>AEEFPVPNGFESAYREVDGVKLHYVKGGQGPLVMLVHGFGQTWYEWHQLMPELAKRFTVIAPDLPGLGQSEPPKTGYSGEQVAVYLHKLARQFSPDRPFDLVAHDIGIWNTYPMVVKNQADIARLVYMDAPIPDARIYRFPAFTAQGESLVWHFSFFAADDRLAETLIAGKERFFLEHFIKSHASNTEVFSERLLDLYARSYAKPHSLNASFEYYRALNESVRQNAELAKTRLQMPTMTLAGGGHGGMGTFQLEQMKAYAEDVEGHVLPGC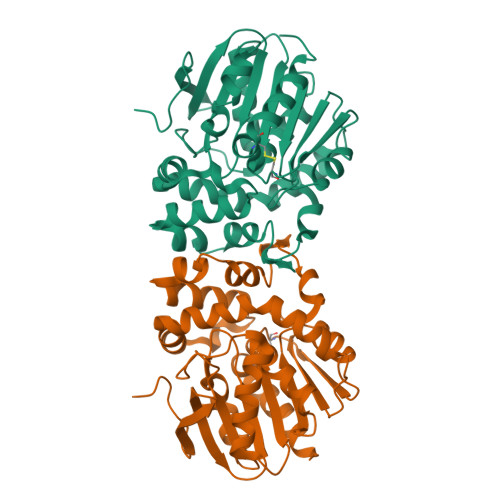GHWLPEECAAPMNRLVIDFLSRGRHHHHHH[4x]>MSQSQRSTADWQRLDAAHHLHPFTDYGELNTKGSRIITRAEGCYLWDSDGNQILDGMAGLWCVNIGYGRKELAEVAYRQMQELPYYNNFFQCSHPPAIELSRLLSEVTPKHMNHVFFTGSGSDSNDTILRMVRYYWKLLGKPYKKVVISRENAYHGSTVAGASLSGMKAMHAQGDLPIPGIEHIEQPYHFGRAPDMDPAEFGRQAAQALERKIDEIGECNVAAFIAEPIQGAGGVIIPPDSYWPEIKRICAERDILLIVDEVITGFGRLGTWFGSQYYDLQPDLMPIAKGLSSGYMPIGGVMVSDRVAKVVIEEGGEFFHGYTYSGHPVAAAVAAENIRIMRDEGIIERAGAEIAPYLQARWRELGEHPLVGEARGVGMVAALELVKSKQPLERFEEPGKVGSLCRDLSVKNGLVMRAVGGTMIISPPLVLSREQVDELIDKARRTLDETHKAIGGALEHHHHHH[4x]

Herein we present the development of a PluriZyme, TR2E2, with efficient native transaminase (k cat: 69.49±1.77 min−1) and artificial esterase (k cat: 3908–0.41 min−1) activities integrated into a single scaffold, and evaluate its utility in a cascade reaction. The reaction proceeds through the conversion of the β‐keto ester into the β‐keto acid at the hydrolytic site and subsequently into the β‐amino acid (e.e. >99 %) at the transaminase site. In addition, we report the crystal structures of the TR2 enzyme and the newly designed TR2E2 PluriZyme. It presents the typical type I fold of class III ω‐TA observed in known structures present in the PDB database, and it contains the characteristic pyridoxal‐5′‐phosphate (PLP)‐binding domain composed of β‐sheets and the catalytic base Lys289.

We aimed to crystalize and solve the structure of TR2. The obtained crystals were optimized in 24‐well sitting drop crystallization plates. The crystals of TR2 diffracted moderately, and a dataset was collected at 3.6 Å resolution (statistics for the data are presented in Table S1). The TR2 crystals were phased by molecular replacement using PHASER in the Phenix program, and a model calculated with AlphaFold as a template. TR2 shows an asymmetric unit of four peptide chains building a functional dimer. The TR2 monomer is subdivided into a core domain, which is the PLP‐binding domain, and a C‐terminal subdomain. The core domain is composed of a central β‐sheet consisting of the strands β1–β7 surrounded by helices α1–α2 and the short helical structures η1 and η2. The smaller subdomain at the C‐terminus consists of the three α‐helices and β‐strands 8, 9, and 10. TR2 is a functional dimer, as represented by Figure 1B; here, the tunnel for accessing the binding pocket with the catalytic base (red circle) is composed of the two monomers (highlighted in different colors). TR2 showed maximal transaminase activity at 45–55 °C, suggesting that it is moderately thermostable. Interestingly, TR2E2 was designed using a site where a loop was missing in the crystal structure of the original transaminase TR2; the loop contained one mutation and was modeled with Prime and refined through MD simulations.>[2x]SNAIRDISSIELIKEMRFGWNLGNTLDAECTSWMDYEKNPIGSETCWGNVKTNEDIFKTLMDNQFNVFRIPTTWTGHIGEAPEYKINEQWMKRVHEIVDYPYKNGAFVILNIHHETWNHAFAETVDEAKVELAQVWKQIAEEFKGYGERLIFEGQNAPRKNGTPVEWNGGDKEGWDVVNAMNAVFLETVRSSGGNNAKRHLMIPPYAAACNENSFKNFDFPEDDDKVIASVHAYSPYNFALNNGEGA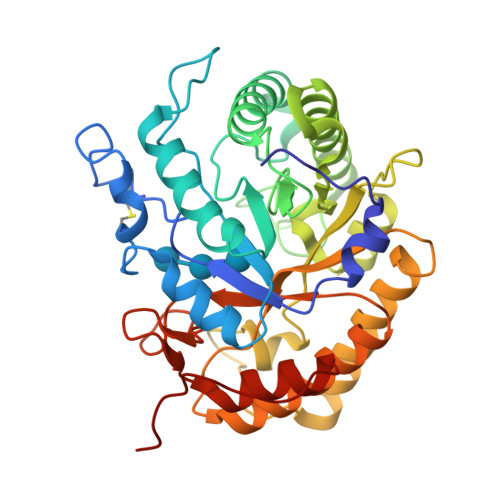VDKFDASGKNELDWNINLMKKRFVDQGIPMILGEYGAMNRDNEEERAAWAEYYMEKITALGVPQVWWDNGVFEGEGERFGLIDRKNLKIVYPSIVAALQKGRGLEVNVLHAIETEPEE>GGSSQKQMSKKMNDQLELMESNIRRDIRQGFVDLQTEKSDLIDNVGAIPFLDYKHFASRIFFPEAGTLTAVMIRDIGEDSEQTTVDEKCLAFAELIRDKQFLSCFVHALEEQKNFSIKDKCTVASLLTLALHGDLLYLTEIMEDLLQSLMDQSSNANPKLLLRRTESIVEKLLTNWMSICLYGFLRESVGQPLFLLVSALTQQISKGPVDSVTEKALYTLSEDWLLCQAQDFEPLKLKVVFAVGTGEEISESLEVIALTCDTIQQVKEKILQTFQRKFGFRYTQQIRDIEIEYEKEGKFVMLQEVDDTSEIRGHVTMLNTLKHYQVGDGACIKVITPKIHAPLKTQNSVKDDKNFSIKYFHLVDPDIDTDLSNHPEKKALKIKEMYLIKLLSTKVAVHSFVENLFKSIWGLPNNKAPLAVKYFFDFLDEQAERKKITDPDVLHIWKTNSLPLRFWVNILKNPDFVFSDMEKSPHLDGCLSVIAQAFMDSFSLTDTHLDKHSPTNKLLYGKDIPQYKQEVKSYYKLVKDQTSISSQELKTFLQEESKKHQNEFNESAALRELYKYMQRYFTEIFQKLEQTDAPSNLKENMHRVKELFDNM[4x];>[4x]GPHMREYKLVVLGSGGVGKSALTVQFVQGIFVEKYDPTIEDSYRKQVEVDAQQCMLEILDTAGTEQFTAMRDLYMKNGQGFALVYSITAQSTFNDLQDLREQILRVKDTDDVPMILVGNKCDLEDERVVGKEQGQNLARQWNNCAFLESSAK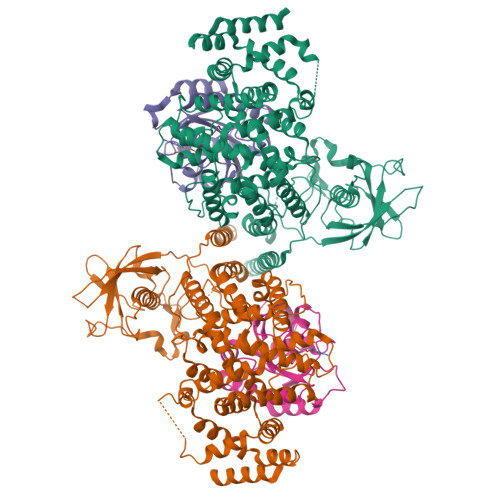SKINVNEIFYDLVRQINSGGSGSGSSGGSGSGGGSGSGSSGLPETGG The initial structural studies revealed GALE requires tightly, non-covalently bound nicotinamide adenine dinucleotide (NAD+) co-factor for catalytic activity and also established the enzyme as part of the short chain dehydrogenase/reductase (SDR) superfamily. Such proteins are characterized by a conserved Y-X-X-X-K catalytic motif and a signature G-X-X-X-G-X-G motif for co-factor binding. As outlined, AnGALE was able to interconvert between UDP-Glcp and UDP-Galp in vitro resulting in a 75:25 (UDP-Glcp:UDP-Galp) mixture regardless of which substrate was employed (reverse reaction not shown). The overall activity profile for wild-type AnGALE towards UDP-Glcp/UDP-Galp and UDP-GlcpNAc/UDP-GalpNAc interconversion more closely resembles that of EcGALE.

To this end, we have determined the ternary crystal structure of AnGALE complexed with NAD+ and UDP-Glcp. AnGALE was found to crystallize in the C2 space group with an asymmetric unit containing the characteristic homodimer previously reported in both the E. coli and Human forms, along with an additional monomer which also forms a dimer through symmetry. The three monomers are nearly identical with backbone root-mean-square deviation (r.m.s.d.) of 0.2, 0.4, and 0.2 Å between monomer A & B, monomer A & C, and monomer B & C, respectively. As can be seen, the structure folds into two domains consisting of an N-terminal motif (M1 - A201, red) and C-terminal motif (G202 - K371, blue). The NAD+ is anchored within this domain directly atop the β-sheet forming one half of the active site which exists in the cleft between the domains. There are a total of 16 hydrogen bonds anchoring the cofactor within the N-terminal portion of the active site cleft. Examination of the structures reveals the models are remarkably similar, the major difference being that AnGALE has an elongated and slightly bent α6 helix along with an additional short α7 helix prior to β6 compared to HGALE. Focusing on the reaction center, Y156, postulated to be the active site base in the Human enzyme (Y157), forms a similar hydrogen bond to the substrate 4'-hydroxyl group (3.4 Å) previously observed in HGALE (3.2 Å). Also of importance to the reaction mechanism is the hydride transfer distance between C4 of the sugar and C4 of the nicotinamide ring which was found to be 3.5 Å in both enzymes.

>[3x]MPSGSVLVTGGTGYIGSFTTLALLEAGYKVVVADNLYNSSAEALNRIELISGKKAEFAQLDVTDEAAFDKVFEAHPDIDSVIHFAALKAVGESGEKPLDYYHVNVYGTICLLRSMVRHNVTNIVFSSSATVYGDATRFPDMIPIPEHCPLGPTNPYGNTKFAIELAITDVINAQRNNAKKAGNETEAAKWNGALLRYFNPAGAHPSGIMGEDPQGVPYNLLPLLAQVATGKREKLLVFGDDYASHDGTAIRDYIHILDLADGHLKALNYLRANNPGVRAWNLGTGRGSTVYEMIRAFSKAVGRDLPYEVAPRRAGDVLNLTSNPTRANTELGWKAQRTLEQACEDLWLWTKNNPQGYRQQPPAELLEQLKK> MEQPII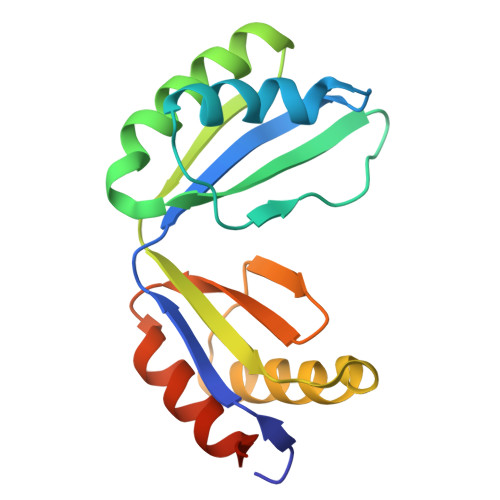SGIAFNRDEAKLTIRGVPDTPGVAFKILGPISAANVEVDMIVQNVAHDNTTDFTFTVHRNDYLNALEILKQTAANIGAREAIGDTNIAKVSIVGVGMRSHAGVASRMFEALAKESINIQMISTSEIKVSVVIEEKYLELAVRALHTAFELDAPARQGE> GSGGSGKVVKFSYMWTINNFSFCREEMGEVIKSSTFSSGANDKLKWCLRVNPKGLDEESKDYLSLYLLLVSCPKSEVRAKFKFSILNAKGEETKAMESQRAYRFVQGKDWGFKKFIRRGFLLDEANGLLPDDKLT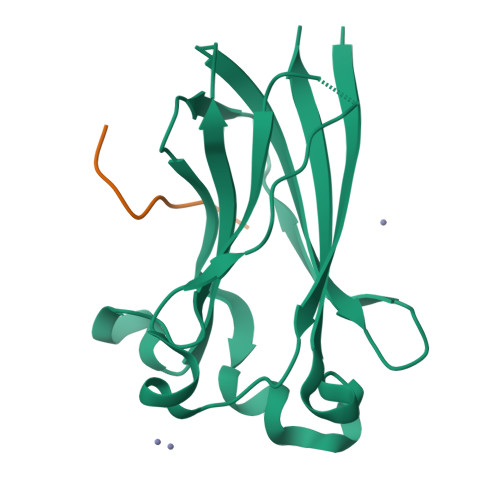LFCEVSVVQD;> KAASADSTTEGTPAD TAR DNA-binding protein 43 (TDP-43) is a ubiquitously expressed RNA-binding protein with diverse roles in RNA processing. The carboxy-terminal part comprises an intrinsically disordered low-complexity domain (LCD), which contains regions enriched in glycine, hydrophobic residues, and glutamine and asparagine (Q/N). The abnormal assembly of TAR DNA-binding protein 43 (TDP-43) in neuronal and glial cells characterizes nearly all cases of amyotrophic lateral sclerosis (ALS) and around half of cases of frontotemporal lobar degeneration (FTLD). Here we report the cryo-electron microscopy structures of assembled TDP-43 from the brains of three individuals with the most common type of FTLD-TDP, type A. TDP-43 formed amyloid filaments with a new fold that was the same across individuals, indicating that this fold may characterize type A FTLD-TDP.

Three-dimensional (3D) classification of the cryo-EM filament segments from the individual with the largest dataset revealed alternative conformations of the N-terminal region R272–G295 and of the turn G335–Q343 linking the fourth and fifth layers. Fewer than 5% of the filament segments contributed to classes with these alternative conformations, demonstrating that they were rare. No variation was observed at regions of zipper packing between β-strands. The alternative conformation of the N-terminal region, but not of the turn linking the fourth and fifth layers, was observed for the second individual, and no alternative conformations were observed for the third individual, consistent with the smaller sizes of their datasets. We determined the structures of filament segments containing the alternative conformations, with resolutions of up to 2.5 Å. In the alternative conformation of the N-terminal region, residues G281–G295 follow approximately the same path as residues R272–P280 in the main conformation, exposing R293 on the filament surface, and residues R272–P280 are in the fuzzy coat. Our mass spectrometry analysis also revealed that R293 was monomethylated in some TDP-43 molecules. Methyl-R293 is incompatible with the main conformation of the filament fold, owing to steric clashes, and can only be accommodated in the alternative conformation of the N-terminal region, where its side chain is exposed. As this alternative conformation is rare, R293 can only be methylated in a minority of TDP-43 molecules. Mapping of the filament segment locations in the micrographs revealed that TDP-43 molecules with different local structural variations could coexist in individual filaments.

>[5x]MSEYIRVTEDENDEPIEIPSEDDGTVLLSTVTAQFPGACGLRYRNPVSQCMRGVRLVEGILHAPDAGWGNLVYVVNYPKDNKRKMDETDASSAVKVKRAVQKTSDLIVLGLPWKTTEQDLKEYFSTFGEVLMVQVKKDLKTGHSKGFGFVRFTEYETQVKVMSQRHMIDGRWCDCKLPNSKQSQDEPLRSRKVFVGRCTEDMTEDELREFFSQYGDVMDVFIPKPFRAFAFVTFADDQIAQSLCGEDLIIKGISVHISNAEPKHNSNRQLERSGRFGGNPGGFGNQGGFGNSRGGGAGLGNNQGSNMGGGMNFGAFSINPAMMAAAQAALQSSWGMMGMLASQQNQSGPSGNNQNQGNMQREPNQAFGSGNNSYSGSNSGAAIGWGSASNAGSGSGFNGGFGSSMDSKSSGWGM> GDLVIASSEPTQQFRSLTNRWMPINSIRVTVNGKRNDLLAQYYIPEDFLSTHAKCAPNTIPFETYVYGKYELEMKFVANGNKFQCGKVIISVKFDSYQADNINTGFQAALSRPHIMLDLS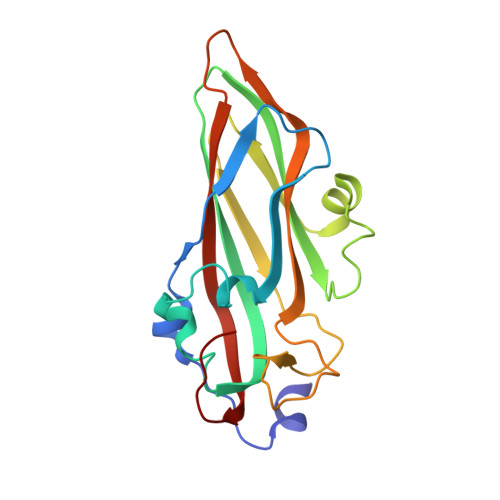TNNEGVLKIPFRYHRAFVRNQTHKTATAGVRPGKFASIYVQVLSPLQTGEGGANDMFIRPFYRYTRAEFAGMSYKVPLT4-fluoro-2-methylphenol | C7 H7 F O | 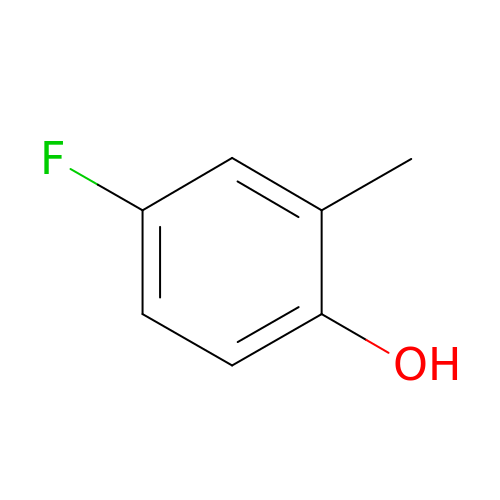GKQDDKKGDIVDAG-UHFFFAOYSA-N>MAHHHHHHMTEATRILLGVNIDHVATLRQARGTRYPDPVKAALDAEEAGADGITVHLREDRRHIQERDVRVLKEVLQTRMNFEMGVTEEMLAFAEEIRPAHSCLVPERREELTTEGGLDVAGQEQRIRDAVRRLAAVGSEVSLFIDPDPRQIEASARVGAPAIELHTGRYADAEDPEEQARELQRVREGVALGRSLGLIVNAGHGLHYHNVEPVA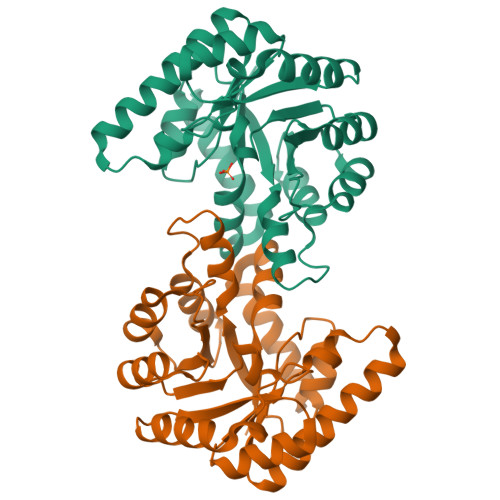AIDGINELNIGHAIVAHALFVGFRQAVAEMKALMLAAATKR[4x]> MLGIPLLTRKAALTPPAPSANPAKIFIRRFFSAGVAKNVVSYSNVMAAQRAMEHPVAFRCLDKLGLTVQSVKWDVGKDPQNTQVGDGGMSASQRKALQQILQRPNPTMSGAQLRYSAALSWACFGRMAFKVSVMSDGSVNAIWPLGIPFLKQKFDRYGDVESFQYGDEAGKETIPSFTKVEKNDKGRPIKNYAFMIVKPSINGAMNFDVQNTPLQAIGVPVALYDALMARAIDSADGTPNSKWLVTASRDLDDGQAKEVKEGIEETKPGGDNGGEIIFIAGTDVKVQEMKNDLSDIHSKVPLDDQARTIAGNFGIPIALLGFAGADGSKFANNYDESRKAFFEDTIEPGYL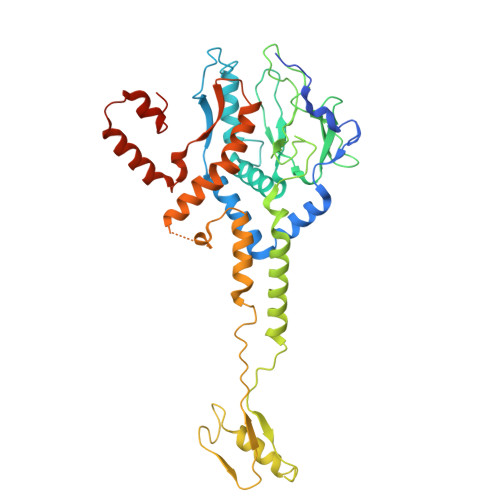TPLEDGFSMFLCGAGYRVIFDRDSIPALRKSRADIAATYDKVTFITEEEKREVTGWPAKKEGQTQNDDA>[2x]GMGRIEVVNVSHIFHRGTPLEKKALENVSLVINEGECLLVAGNTGSGKSTLLQIVAGLIEPTSGDVLYDGERKKGYEIRRNIGIAFQYPEDQFFAERVFDEVAFAVKNFYPDRDPVPLVKKAMEFVGLDFDSFKDRVPFF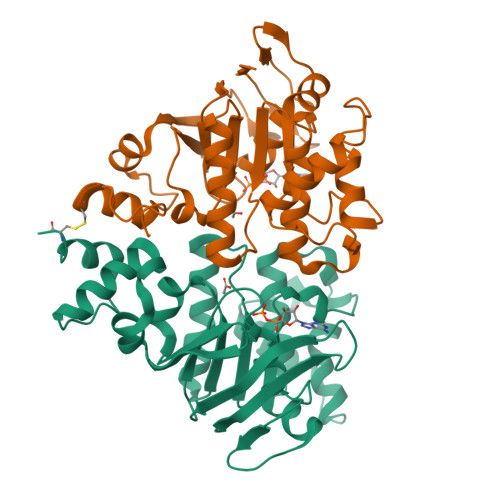LSGGEKRRVAIASVIVHEPDILILDEPLVGLDREGKTDLLRIVEKWKTLGKTVILISHDIETVINHVDRVVVLEKGKKVFDGTRMEFLEKYDPRFFTSKMLVMRRLVLKGEDPFSMSDDELLERVCNS;>[2x]GSGGSHMGSGRIELNSVSFRYNGDYVLKDVNAEFETGKIYVVVGKNGSGKTTLLKILAGLLAAAGEIFLDGSPADPFLLRKNVGYVFQNPSSQIIGATVEEDVAFSLEIMGLDESEMRKRIKKVLELVGLSGLAAADPLNLSGGQKQRLAIASMLARDTRFLALDEPVSMLDPPSQREIFQVLESLKNEGKGIILVTHELEYLDDMDFILHISNGTIDFCGSWEEFVEREFDDVEIPFKWKLWKKCGKINLWEDRYENSGNQRRRDTV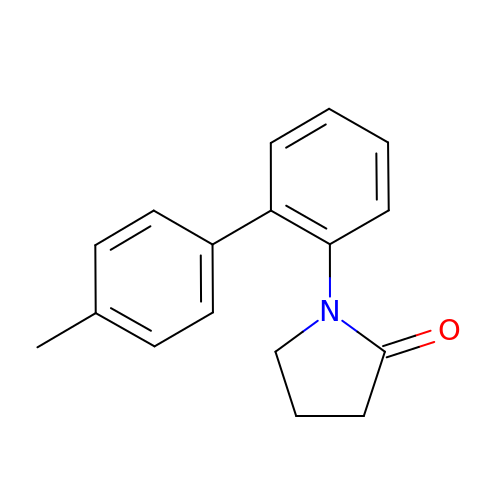1-(4'-methyl[1,1'-biphenyl]-2-yl)pyrrolidin-2-one | C17 H17 N O | YEVWXVKNDBSTQP-UHFFFAOYSA-N>[2x]APLADAALPEPNVFLIFSHGLQGCLEAQGGQVRVTPACNTSLPAQRWKWVSRNRLFNLGTMQCLGTGWPGTNTTASLGMYECDREALNLRWHCRTLGDQLSLLLGARTSNISKPGTLERGDQTRSGQWRIYGSEEDLCALPYHEVYTIQGNSHGKPCTIPFKYDNQWFHGCTSTGREDGHLWCATTQDYGKDERWGFCPIKSNDCETFWDKDQLTDSCYQFNFQSTLSWREAWASCEQQGADLL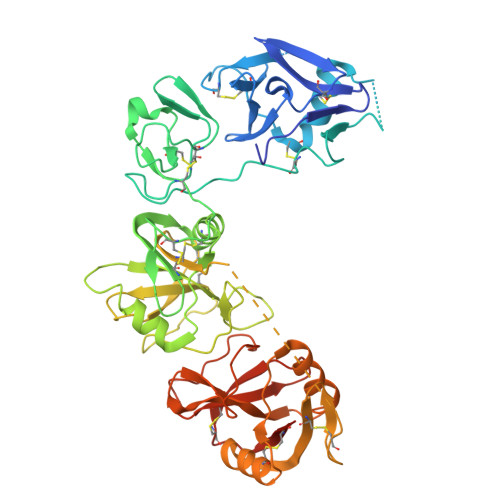SITEIHEQTYINGLLTGYSSTLWIGLNDLDTSGGWQWSDNSPLKYLNWESDQPDNPSEENCGVIRTESSGGWQNRDCSIALPYVCKKKPNATAEPTPPDRWANVKVECEPSWQPFQGHCYRLQAEKRSWQESKKACLRGGGDLVSIHSMAELEFITKQIKQEVEELWIGLNDLKLQMNFEWSDGSLVSFTHWHPFEPNNFRDSLEDCVTIWGPEGRWNDSPCNQSLPSICKKAGQLSGAAAHHHHHH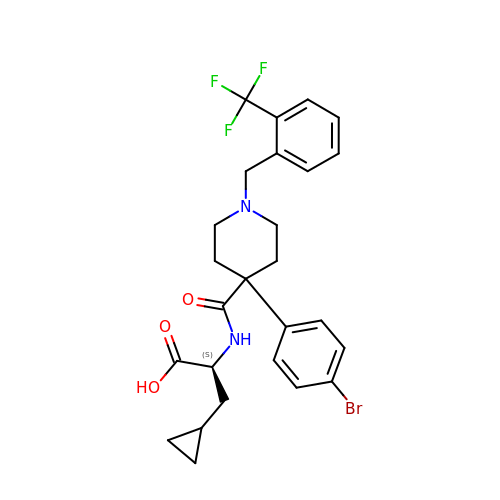N-[4-(4-bromophenyl)-1-{[2-(trifluoromethyl)phenyl]methyl}piperidine-4-carbonyl]-3-cyclopropyl-L-alanine | C26 H28 Br F3 N2 O3 | XTCYTRMSAWHHGP-QFIPXVFZSA-N Two glycosyltransferases (GTases), SdgB and SdgA, are responsible for the glycosylation of S. aureus SDR proteins such as ClfA and ClfB. SdgB first appends N-acetyl­glucosamine (GlcNAc) moieties onto serine residues (O-glycosylation) within the SDR domain using uridine diphos­phate N-acetylglucosamine (UDP-GlcNAc) as a donor substrate. The subsequent addition of GlcNAc to the glycoproteins is catalyzed by the second enzyme, SdgA, yielding glycosylated SDR proteins in which each SD repeat is decorated with GlcNAc disaccharide moieties. The glycosylation of SDR proteins mediated by SdgA and SdgB protects SDR proteins from degradation by host proteases, thereby circumventing innate immune attack.

Despite the biological significance of these two glycosyltransferases involved in pathogenicity and avoidance of the host innate immune response, their structures and the molecular basis of their activity have not been investigated. This study reports the crystal structures of SdgB and SdgA from S. aureus as well as multiple structures of SdgB in complex with its substrates (for example UDP, N-acetylglucosamine or SDR peptides), products (glycosylated SDR peptides) or phosphate ions. Interestingly, SdgB undergoes a conformational change from an open to closed complex upon substrate binding. In addition to the dimerization role, the inserted domain was found to serve as a binding platform for the SD repeats before and after glycosylation.

>[2x]SMNYFVGNSLGVNLTGIEKAIINRLNLFKEMGRPAQCVFLSWNRYLYRNAQNYITSSDYINMYDFFQEATYLERNEPFDWLSYWTDECHYTLKHVENSHDFRIYDQERFLMYAHFQDPKYRILDYVNHFDSQRRKVKRDFYDVRGFLSCSRILVDKQQTLCEFFYNPEGDTKLEKYFSYKDGKPEVQKIIVYYANKQYFFNNETELGAFFIKQLYQHGDLFFSDRNVYTAPIFNLTPESIPVVAVLHSTHIKNIDALDSSPFKNVYKAMFENLSRYRAIIVSTEQQKLDVEKRINHTIPVVNIPVGYSETIDTPVQTLDQRSVKLISVARYSPEKQLHQQIELIKRLVSYVPKIELHMYGFGSESKKLNELIQKYGLENHVYLRGFLSNLDQEYSDAYLSLITSNMEGFSLALLESLAHGVPVISYDIKYGPNELITSDFNGYLITKNDEDALFDKVKYVIDHPEVQQRLSKGSLAKAQQYSKASLIKQWDQFVRLILEHHHHHH;>DSDSD[2x]> TFFNPDREGWLLKLGGRVKTWKRRWFILTDNCLYYFEYTTDKEPRGIIPLENLSIREVLDPRKPNCFELYNPSHKGQVIK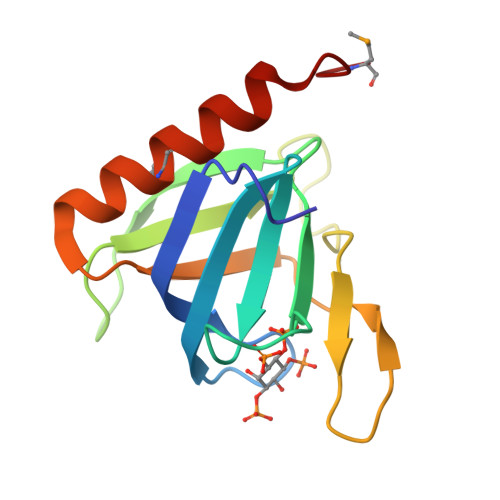ACKTEADGRVVEGNHVVYRISAPSPEEKEEWMKSIKASISRDPFYDM> GSMPKPINVRVTTMDAELEFAIQPNTTGKQLFDQVVKTVGLREVWFFGLQYVDSKGYSTWLKLNKKVTQQDVKKENPLQFKFRAKFFPEDVSEELIQEITQRLFFLQVKEAILNDEIYCPPETAVLLASYAVQAKYGDYNKEIHKPGYLANDRLLPQRVLEQHKLTKEQWEERIQNWH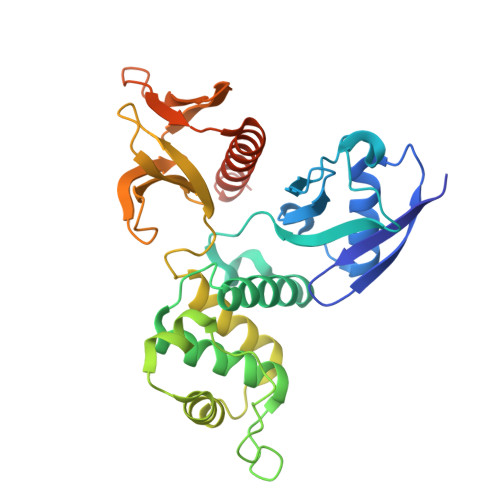EEHRGMLREDSMMEYLKIAQDLEMYGVNYFEIKNKKGTELWLGVDALGLNIYEHDDKLTPKIGFPWSEIRNISFNDKKFVIKPIDKKAPDFVFYAPRLRINKRILALCMGNHELYMRRRKPDTIEVQQMKAQAR> GGTGGGGCATGCCCCACC

Nine new crystal structures of CG-rich DNA 18-mers with the sequence 5′-GGTGGGGGC-XZ-GCCCCACC-3′, which are related to the bacterial repetitive extragenic palindromes, are reported. All 18-mers crystallized as isomorphic tetragonal crystals with one strand of a right-handed antiparallel duplex in the asymmetric unit. All reported structures co-crystallized with the Sr2+ cation located between nucleotides 6 and 7 and (by symmetry) 12 and 13.

All four Chom-18-mers with two central nucleotides (residues 9 and 10) able to form Watson–Crick pairs were crystallized. Base pairs A–T and T–A are classified as Watson–Crick pairs, while the C–G pair adopts a specific orientation characterized by a large value of one of the base parameters, shear (2.97 Å), and is not classified. NtC classes provided valuable help with building the initial models of six of the nine 18-mers, i.e. Chom-18-AT, Chom-18-CG, Chom-18-GC, Chom-18-GT, Chom-18-TC and Chom-18-AG.> GHMASMAKIKNQYYNESVSPIEYAQQGFKGKMRSVNWNVVNDEKDLEVWNRITQNFWLPEKIPVSNDLTSWRTLTPEWQELITRTFTGLTLLDTIQATVGDVAQVPNSLTDHEQVIYTNFAFMVAVHARSYGSIFSTLCSSEQIEEAHEWVINTETLQERAKALIPYYVNDDPLKSKVAAALMPGFLLYGGFYLPFYLSARGKLPNTSDIIRLILRDKVIHNYYSGYKYQKKVAKLSPEKQAEMKEFVFKLLYELIDLEKAYLKELYEDFGLADDAIRFSVYNAGKFLQNLGYDSPFTEEETRIEPEIFTQLSARADENHDFFSGNGSSYIMGVSEETEDDDWEF

Aerobic RNR (class I) depends on the ferritin-like R2 subunit to generate a catalytic radical in an oxygen dependent reaction; the radical must be transferred back-and-forth with the catalytic R1 subunit, which performs the ribonucleotide reduction. Radical translocation between the subunits proceeds via reversible long-range proton-coupled electron transfer (PCET) in a transient R1-R2 complex. In a recently discovered active metal-free R2 subclass, denoted R2e, this tyrosine residue is post-translationally meta-hydroxylated to a 3,4-dihydroxyphenylalanine (DOPA) which serves as the radical-harboring residue. From an experimental point of view, R2e from Mesoplasma florum (MfR2) represents an attractive model to study active radical states in RNRs.

To circumvent photoreduction artefacts, we used XFEL serial femtosecond crystallography to determine the structure of the catalytically active radical state of MfR2 at atomic resolution. The active radical-harboring protein was crystallized in batch to produce a suspension of blue microcrystals used to collect room temperature serial femtosecond diffraction data at an XFEL source. The resulting dataset produced a model of the protein at 1.5 Å resolution, and the electron density map allows unambiguous interpretation. A short H-bond between DOPAY126 meta-O and D88 is present with a O–O distance calculated to 2.41 ± 0.05 Å using END/RAPID error analysis. A striking conformational shift takes place upon radical acquisition between DOPAY126 and D88: the dyad undergoes a coupled coplanar (but not coaxial) rotation of ~22°, with an additional rotation of the aromatic ring of ~12° along the Cβ-C1 axis. It results in a 2-Å displacement of the para-O carrying the main radical spin density, away from D88, and a reorganization of the interaction pattern around DOPAY126. In addition, a clearly defined water molecule (w1) mediates a new H-bond between DOPAY126 and the ε-ammonium group of K213, which displays a different orientation facing towards DOPAY126. In contrast, in the radical state of MfR2, this water network is disrupted by Q91 which undergoes a large sidechain flip towards D88. Our data suggest that Q91 could play a key role as it obstructs the putative oxidant channel in the radical state, preventing radical quenching by further oxidant access to the active site. In the immediate vicinity of the side chain of DOPAY126, residues L183 and F187 undergo large conformational changes in the radical state of MfR2, leaving space for the positioning of three water molecules (including w1) and creating a water-mediated H-bond network between DOPAY126, D88, K213 and Q91.> 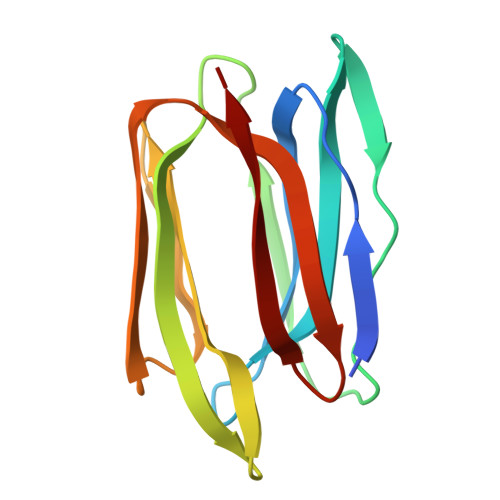STSSNGKAFDDGAFTGIREINLSYNKETAIGDFQVIYDLNGSPFVGQNHTSFITGFTPVKISLDFPSEYIIEVSGHTGKVSGYVVVRSLAFKTNKKTYGPYGVTSGTPFNLPIENGLIVGFKGSIGYWLDYFSMYLSL> HGMSQPACTARRRTRVLILGVNGFIGNHLTERLLREDHYEVYGLDIGSDAISRFLNHPHFHFVEGDISIHSEWIEYHVKKCDVVLPLVAIATPIEYTRNPLRVFELDFEENLRIIRYCVKYRKRIIFPSTSEVYGMCSDKYFDEDHSNLIVGPVNKPRWIYSVSKQLLDRVIWAYGEKEGLQFTLFRPFNWMGPRLDNLNAARIGSSRAITQLILNLVEGSPIKLIDGGKQKRCFTDIRDGIEALYRIIENAGNRCDGEIINIGNPENEASIEELGEMLLASFEKHPLRHHFPPFA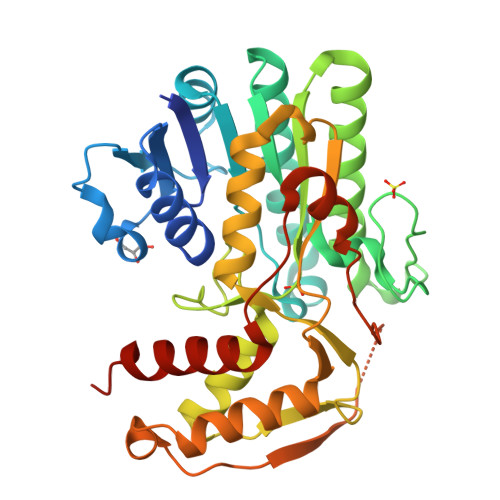GFRVVESSSYYGKGYQDVEHMKPSIRNAHRCLDWEPKIDMQETIDETLDFFLRTVDLTDKPS3-(3,4-DIMETHOXYPHENYL)PROPIONIC ACID | C11 H14 O4 | 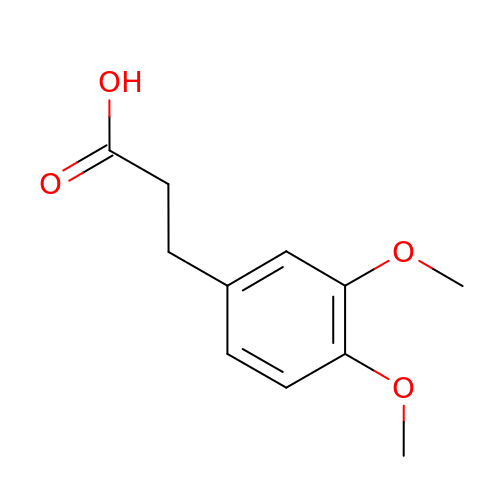LHHKQWQTBCTDQM-UHFFFAOYSA-N>[2x]GPPAVVATRVPPTHAALRRPTIELEFDRAIEPGSVPHIVLRADDGTSVAVGPLSWLSDRRIAFAPRKPLKSNSRYEIMVPAGIRSTTGERSTHPLTSSFDTAPVTPPRGLPNLDGASCFINTALQLAVHSSALDDILSNEAVPPAVRTLLEDYDAASADALDAQLAAAVAALRATPEVPDSGPGQTLEVMQALRMPLYDTSSANNAKNNADAIRHAPPNTKAFFLNSYPPLSYA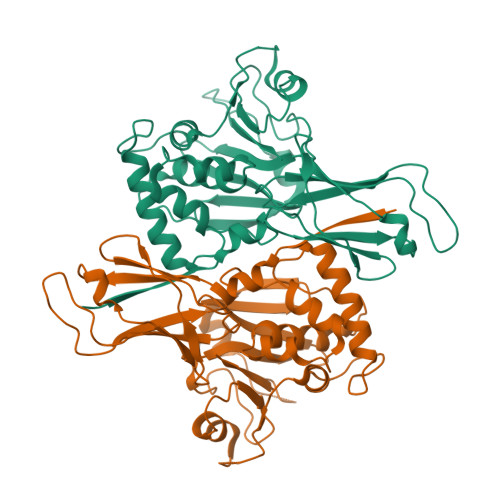DLPNHDRLVAFDYSTGGHYVAYVKRDGIWYRIDDAQVSAVNEQDLLALPAFNPANGSVSIEIAIYR>[4x]MLKQVEIFTDGSCLGNPGPGGYGAILRYRGREKTFSAGYTRTTNNRMALMAAIVALEALKEHCEVILSTDSQYVRQGITQWIHNWKARGWKTADKKPVKNVDLWQRLDAALG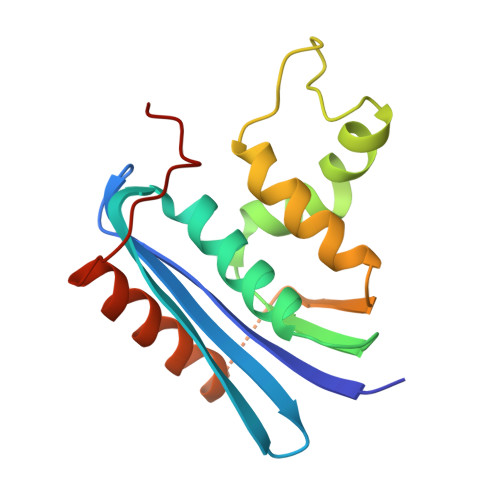QHQIKWEWVKGHAGHPENERCDELARAAAMNPTLEDTGYQVEV>MPSTPEEKKKVLTRVRRIRGQIDALERSLEGDAECRAILQQIAAVRGAANGLMAEVLESHIRETFDRNDCYSREVSQSV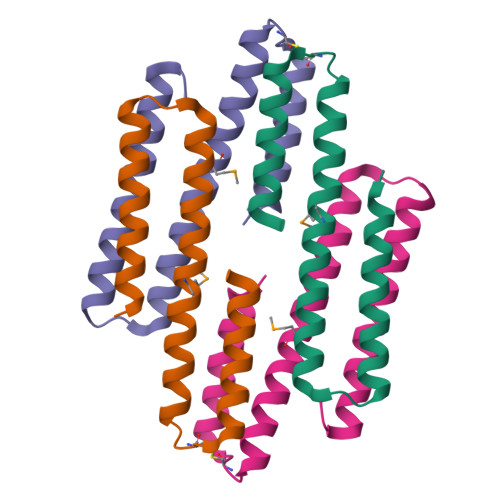DDTIELVRAYLK[4x]>[4x]HHMSAIKPDMKINLRMEGNVNGHHFVIDGDGTGKPFEGK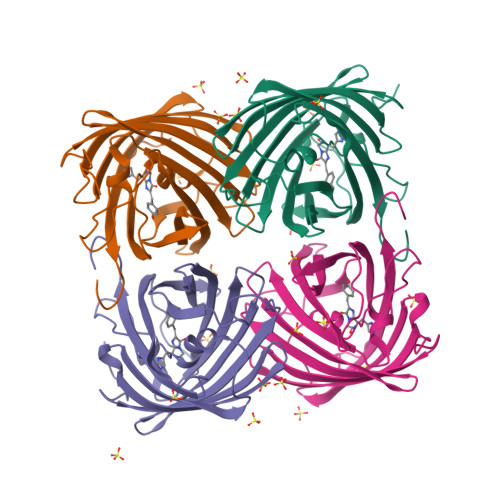QSMDLEVKEGGPLPFAFDILTTAFHYGNRVFAEYPDHIQDYFKQSFPKGYSWERSLTFEDGGICIARNDITMEGDTFYNKVRFHGVNFPANGPVMQKKTLKWEPSTEKMYVRDGVLTGDITMALLLEGNAHYRCDSRTTYKAKEKGVKLPGYHLVDHCIEILSHDKDYNKVKLYEHAVAHSGLPDN> AGPWADIMQGPSESFVDFANRLIKAVEGSNLPPSAR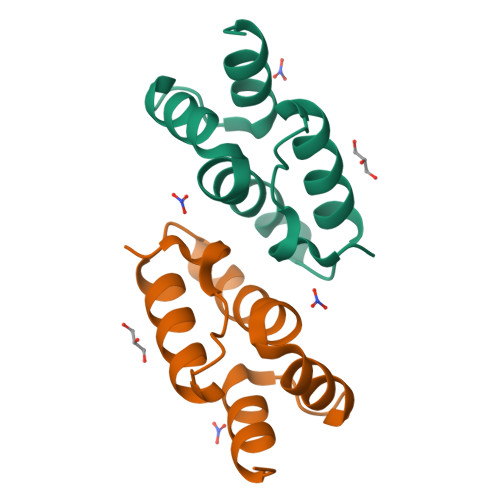APVIIDCFRQKSQPDIQQLIRTAPSTLTTPGEIIKYVLDRQ> MRDEEPVRRLETIVEEERRVVVQGYVFDAEVSELKSGRTLLTMKITDYTNSILVKMFSRDKEDAELMSGVKKGMWVKVRGSVQNDTFVRDLVIIANDLNEIAANERQDTAPEGEKRVELHLHTPMSQMDAVTSVTKLIEQAKKWGHPAIAVTDHAVVQSFPEAYSAAKKHGMKVIYGLEANIVDDGVPIAYNETHRRLGSGSGPFHVTLLAQNETGLKNLFK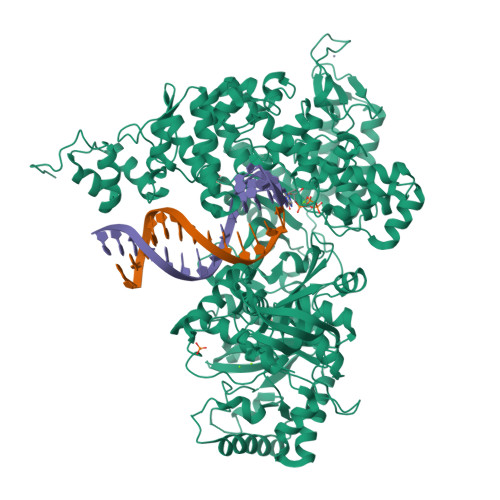LVSLSHIQYFHRVPRIPRSVLVKHRDGLLVGSGCDKGELFDNLIQKAPEEVEDIARFYDFLEVHPPDVYKPLIEMDYVKDEEMIKNIIRSIVALGEKLDIPVVATGNVHYLNPEDKIYRKILIHSQGGANPLNRHELPDVYFRTTNEMLDCFSFLGPEKAKEIVVDNTQKIASLIGDVKPIKDELYTPRIEGADEEIREMSYRRAKEIYGDPLPKLVEERLEKELKSIIGHGFAVIYLISHKLVKKSLDDGYLVGSRGSVGSSFVATMTEITEVNPLPPHYVCPNCKHSEFFNDGSVGSGFDLPDKNCPRCGTKYKKDGHDIPFETFLGFKGDKVPDIDLNFSGEYQPRAHNYTKVLFGEDNVYRAGTIGTVADKTAYGFVKAYASDHNLELRGAEIDRLAAGCTGVKRTTGQHPGGIIVVPDYMEIYDFTPIQYPADDTSSEWRTTHFDFHSIHDNLLKLDILGHDDPTVIRMLQDLSGIDPKTIPTDDPDVMGIFSSTEPLGVTPEQIMCNVGTIGIPEFGTRFVRQMLEETRPKTFSELVQISGLSHGTDVWLGNAQELIQNGTCTLSEVIGCRDDIMVYLIYRGLEPSLAFKIMESVRKGKGLTPEFEAEMRKHDVPEWYIDSCKKIKYMFPKAHAAAYVLMAVRIAYFKVHHPLLYYASYFTVRAEDFDLDAMIKGSAAIRKRIEEINAKGIQATAKEKSLLTVLEVALEMCERGFSFKNIDLYRSQATEFVIDGNSLIPPFNAIPGLGTNVAQAIVRAREEGEFLSKEDLQQRGKLSKTLLEYLESRGCLDSLPDHNQLSLFSGGHHHHHHHH> GSM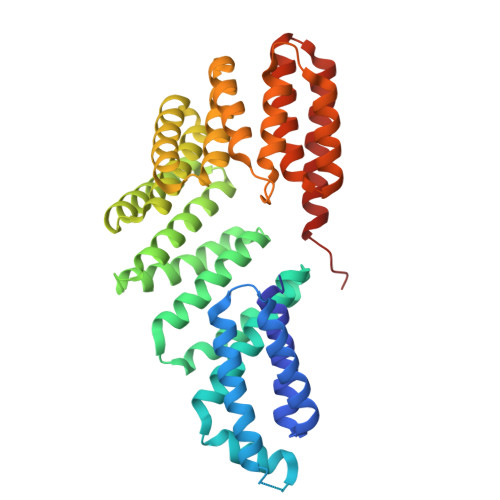SQAIPSSRVGVKINEWYKMIRQFSVPDAEILKAEVEQDIQQMEEDQDLLIYYSLMCFRHQLMLDYLEPGKTYGNRPTVTELLETIETPQKKLTGLLKYYSLFFRGMYEFDQKEYVEAIGYYREAEKELPFVSDDIEKAEFHFKVAEAYYHMKQTHVSMYHILQALDIYQNHPLYSIRTIQSLFVIAGNYDDFKHYDKALPHLEAALELAMDIQNDRFIAISLLNIANSYDRSGDDQMAVEHFQKAAKVSREKVPDLLPKVLFGLSWTLCKAGQTQKAFQFIEEGLDHITARSHKFYKELFLFLQAVYKETVDERKIHDLLSYFEKKNLHAYIEACARSAAAVFESSCHFEQAAAFYRKVLKAQEDILKGECLYAY>[2x]GHMGPNAVELTTDQAWCLADVLGAGSYPW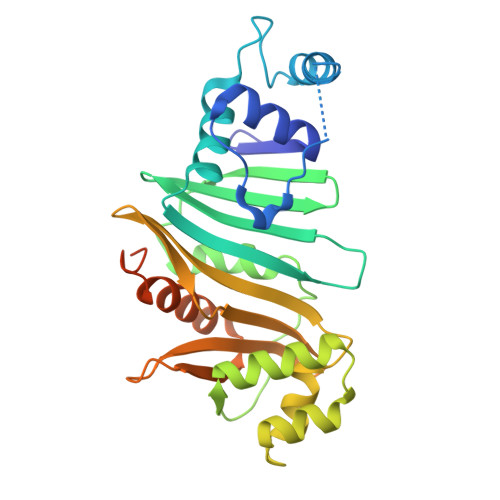VLAITPPYSDHSQRSAFLAAQSAELTRMGVVNSAGAVDPRVAQWITTVCRATQWLDLRFVSGPGDLLRGMVARRSEETVVALRNAQLVTFTAMDIGHQHALVPVLTAGLSGRKPARFDDFALPAAAGARADEQIRNGAPLAEVLEFLGVPPSARPLVESVFDGRRTYVEIVAGEHRDGHRVTTEVGVSIIDTPHGRILVHPTKAFDGEWISTFTPGSADAIAMAVERLTASLPSGSWFPDQPLTRDFDEDAATHREPVLQRRTQKA>[2x]MASGSAS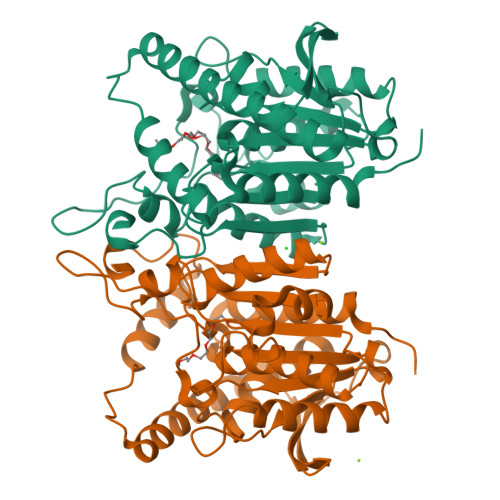SAQTPGLMSWLPPSNQLSPEARSVLDRMDAAKAPEFNGDLVRQRAFYQQFNDDRLVEMRRVFRTRERHETLNAVHVQVVEPADGVSARNRDRVLINVHGGAFMWGAGSGALVEAIPIAATMGVSVVTVDYRLAPENRYPAASEDVTAVYRALLERYPAANIGIFGTSAGGVITAQAVTWIRREGLPRPGAIGTLSGTGAPYSGDSPYLAGVVPVGPGVKAPPLPGLLPTAYMEGVGADDARAYPLTSDAETVFMPPTLLLAGGRDFAVSALSLAHRRLARAGVDSELHLFDGLPHAFFVWPDMPESLEAYALIAGFFDSRLGLTPSSSIPTPRSPSLEHHHHHH>[2x]ARTKQTIHPGVTCDGCQMFPING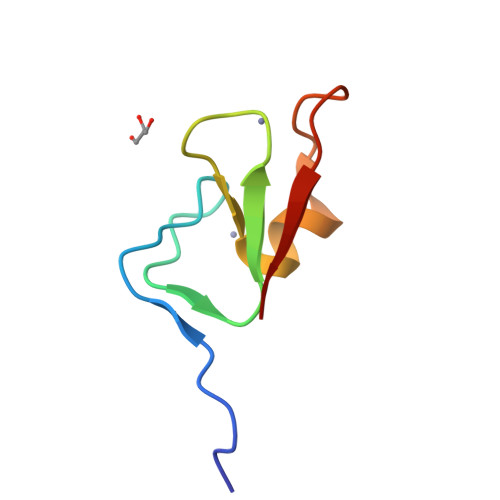SRFKCRNCDDFDFCETCFKTKKHNTRHTFGRIN[(1S,3S,5R,6R,8R)-6-(6-AMINOPURIN-9-YL)-4'-ETHYLAMINO-3'-FLUORO-SPIRO[2,4,7-TRIOXA-3-BORANUIDABICYCLO[3.3.0]OCTANE-3,7'-8-OXA-7-BORANUIDABICYCLO[4.3.0]NONA-1,3,5-TRIENE]-8-YL]METHYL DIHYDROGEN PHOSPHATE | C19 H22 B F N6 O8 P | 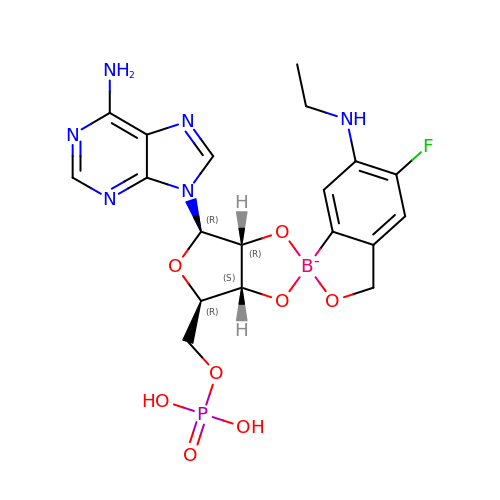KLENTOAZKNOXCI-JNRNKGNBSA-N2,2-dimethylpropyl 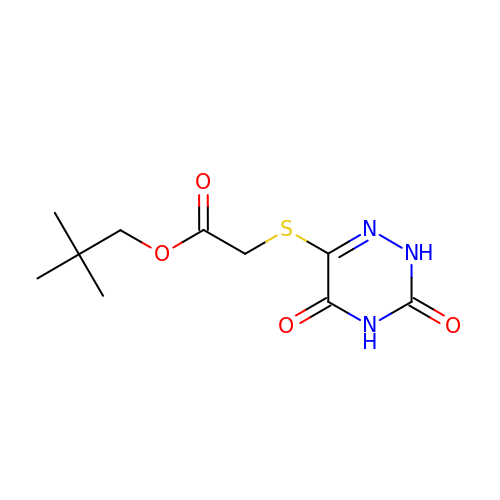2-[[3,5-bis(oxidanylidene)-2~{H}-1,2,4-triazin-6-yl]sulfanyl]ethanoate | C10 H15 N3 O4 S | HHKUCSHMOMLQAX-UHFFFAOYSA-N4-[3-cyclohexyl-5-(4-fluorophenyl)imidazol-4-yl]-1~{H}-pyrrolo[2,3-b]pyridine | C22 H21 F N4 | 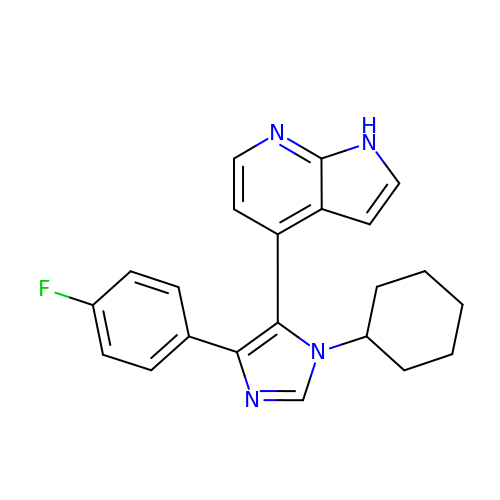CPDVWRAEVIUDHW-UHFFFAOYSA-N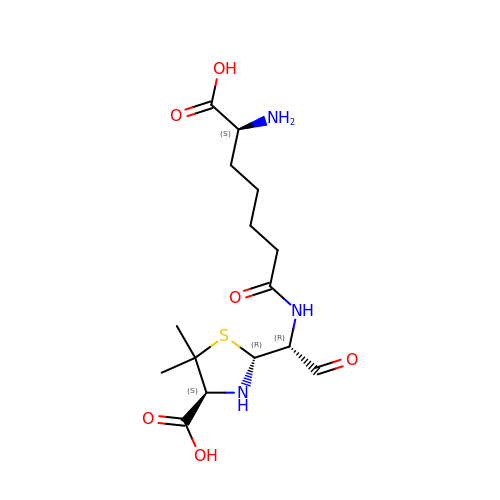(2R,4S)-2-[(1R)-1-{[(6S)-6-amino-6-carboxyhexanoyl]amino}-2-oxoethyl]-5,5-dimethyl-1,3-thiazolidine-4-carboxylic acid | C15 H25 N3 O6 S | AEEFBHZTXIEBJN-BSJXLVFVSA-N> EMAESVTNPQ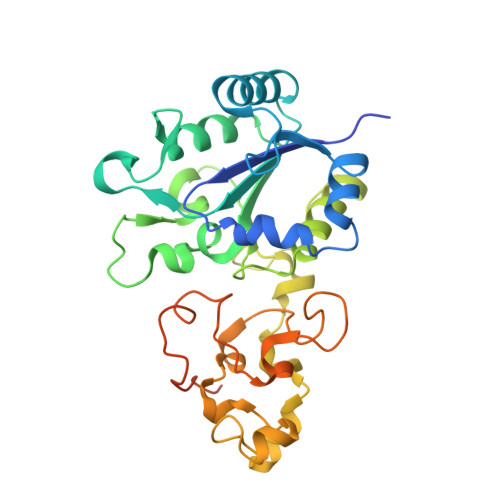RPPVIWIGAQECTGCTESLLRATHPTVENLVLETISLEYHEVLSAAFGHQVEENKHNALEKYKGQYVLVVDGSIPLKDNGIYCMVAGEPIVDHIRKAAEGAAAIIAIGSCSAWGGVAAAGVNPTGAVSLQEVLPGKTVINIPGCPPNPHNFLATVAHIITYGKPPKLDDKNRPTFAYGRLIHEHCERRPHFDAGRFAKEFGDEGHREGWCLCHLGCKGPETYGNCSTLQFCDVGGVWPVAIGHPCYGCNEEGIGFHKGIHQLANVENQTPRSQKPDVNAKEGGNVSRSHHHHHH> SMAEPLKEEDGEDGSAEPPGPVKAEPAHTAASVAAKNLALLKARSFDVTFDVGDEYEIIETIGNGAYGVVSSARRRLTGQQVAIKKIPNAFDVVTNAKRTLRELKILKHFKHDNIIAIKDILRPTVPYGEFKSVYVVLDLMESDLHQIIHSSQPLTLEH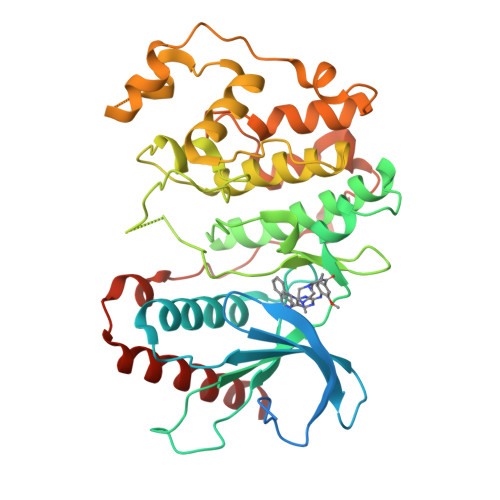VRYFLYQLLRGLKYMHSAQVIHRDLKPSNLLVNENCELKIGDFGMARGLCTSPAEHQYFMTEYVATRWYRAPELMLSLHEYTQAIDLWSVGCIFGEMLARRQLFPGKNYVHQLQLIMMVLGTPSPAVIQAVGAERVRAYIQSLPPRQPVPWETVYPGADRQALSLLGRMLRFEPSARISAAAALRHPFLAKYHDPDDEPDCAPPFDFAFDREALTRERIKEAIVAEIEDFHARREGIRQ>[2x]GHMSNVSALPLQPGTTPSGGGSVRDRVSPQEWEVRVKLAAAYRLAALKRWTDHIYTHFSARVPGPDEHFLINAFGLLFDEITASNLVKVDIDGTIVDDPTGLGINYAGYVIHSAIHAARHDLQAVLHTHTRDGIAVSAQKDGLLPISQHSIAFSGRVAYHGYEGIALDLSERERLV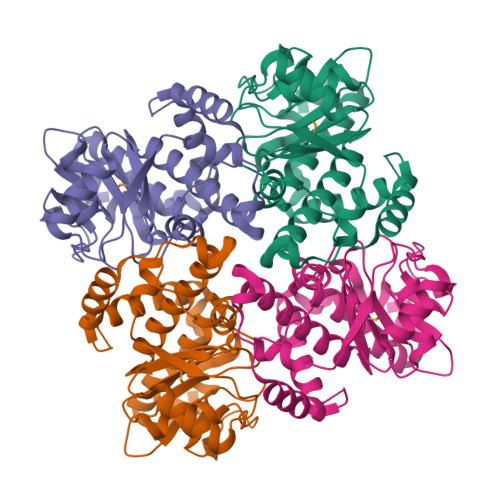ADLGDKSVMILRNHGLLTGGVSVEHAIQQLHALEYACNIQIAAQSAGNAELVFPPREVIAKVEEQAKAIKDGNGPGVARHWNALIRELERSGTDYRD Shewanella species produce hydroxamate-type siderophores and iron removal from these compounds can occur in the cytoplasm via Fe(III)–siderophore reduction mediated by siderophore-interacting proteins (SIPs). SIPs contain stably attached flavins and use NADH and/or NADPH as reducing agents. As a result, these two enzyme families are considered to have a redundant role: reducing ferric iron complexed with siderophores to its ferrous form, which decreases the complex’s affinity and facilitates iron release. Here, we present the functional characterization and structure determination of a novel SIP from S. bicestrii (SbSIP) and show that it is an NAD(P)H–siderophore oxidoreductase.

The structure of SbSIP was determined at 1.9 Å resolution. The structure revealed two domains as previously described for other SIPs: a N-terminal or NAD(P)H binding domain and a C-terminal or FAD binding domain. The NAD(P)H binding domain consists of the typical β1–α1–β2 Rossmann fold architecture composed of a manifold of β-antiparallel-strands (β1–β6) and two short α-helices (α1 and ƞ1). The FAD binding domain is composed of five antiparallel β-strands (β7–β11) with two short α-helices (α2 and α3) connected by long loops. The FAD isoalloxazine ring shows a planar conformation and is stabilized through aromatic stacking interactions with Tyr-60 and Tyr-225, and hydrogen bonds with residues Thr-61 (backbone O and N), Tyr-59 (side chain OH), Val-75 (backbone N), and Asp-73 (backbone O). The negatively charged phosphate groups of FAD are also stabilized through hydrogen bonds with Thr-60 (backbone N), Glu-232 (backbone N), His-77 (side chain Nε2), Gly-81 (backbone N), Ser-84 (Side chain OH), and Ala-83 (backbone N). The triad of basic amino acid residues (Lys-45, Lys-236, and Lys-239 reported in SIP from S. putrefaciens, SpSIP) and proposed to form the Fe(III)–siderophore binding pocket is well conserved (Lys-44, Lys-236, and Lys-239 in SbSIP). As previously observed for SpSIP, Lys-44 forms a ridge with Lys-236, making the access to the FAD cofactor smaller when compared to SfSIP. However, the pocket of SbSIP is substantially smaller when compared to SfSIP. However, the access pocket to the FAD cofactor is smaller than in the case of SfSIP and likely sets the preference for NADH via steric clash with the 2′ phosphate group of NADPH.

>[2x]MNRPAPRELTVIGKTQVTPHMLRITLGGAGFAGFPADQESAYIKLLFPQQGDERPLMRTYTIRQQRMNEIDVDFVLHDTDGPASRWAKSTEIGDTIQIGGPGLKKLINLNAEWFLLAGDMTALPAISVNLTQLPNNAVGYAVIEVLSEADIQPLVHPRNVQLHWVINPEADPEGKPLAERIAQLPKLEGQGAVWLACEFSSMRALRKLLKQTYDLPKSHFYTSSYWKIGCNEGEHKLVKQQDEQLENNTVG>[2x]SNAEDELPVKGISNLNNMAMFSVSGPGMKGMVGMAARVFAAMSRARISVVLITQSSSEYSISFCVPQSDCVRAERAMQ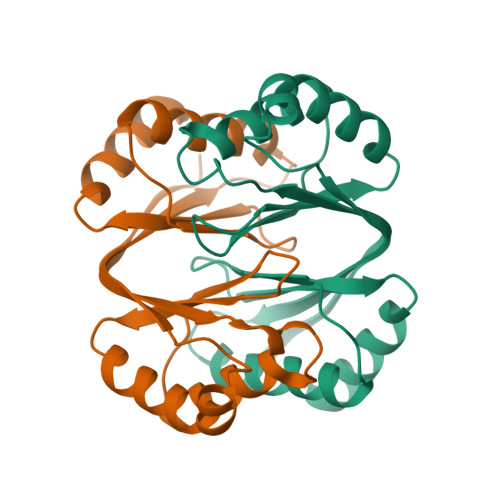EEFYLELKEGLLEPLAVTERLAIISVVGDGMRTLRGISAKFFAALARANINIVAIAQGSSERSISVVVNNDDATTGVRVTHQMLF7-(2-methoxyethoxymethyl)-1,3-dimethyl-purine-2,6-dione | C11 H16 N4 O4 | 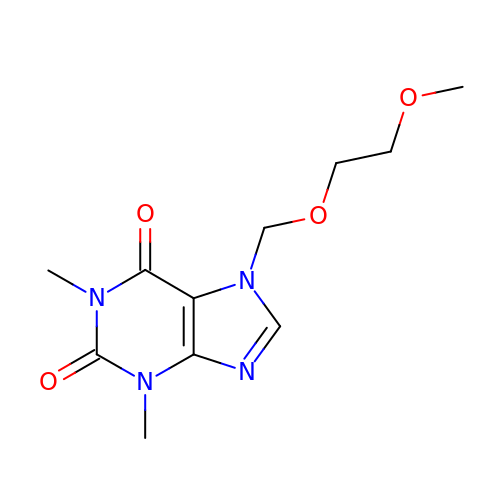BSIZPWZVMIVPIN-UHFFFAOYSA-N Using an ambisense coding strategy, LASV genome encodes four proteins: glycoprotein complex (GPC), nucleoprotein (NP), matrix protein (Z), and the L RNA-dependent RNA polymerase. Instead, these viruses steal the caps from host mRNAs in a process termed cap snatching. In arenaviruses, mutagenesis studies have revealed that the N-terminal domain of the LASV L protein, which consists of 250 amino acid residues, is uniquely required for viral transcription but not replication, implicating its potential role in cap snatching. Our work confirms that arenavirus L polymerase proteins contain a conserved endonuclease domain at the N-terminal region.

Toward this end, we report here for the first time the crystal structure of the endonuclease domain of the LASV L protein in complex with Mg2+ ions at 1.72 Å and demonstrate its enzymatic activity required for viral RNA transcription. The final protein product for crystallization consists of residues 1–173 based on the structure determined. The protein contains an N-terminal domain that consists of a four α-helices bundle (α1, α2, α3 and α7) and a C-terminal domain that composes of three antiparallel β-sheets (β1, β2 and β3) and two helices (α4 and α5). Between the two domains is a highly positively charged groove, which we speculate to be a RNA binding site, and a highly negatively charged cavity, which harbors two magnesium ions (Mg2+) and is a potential active site of the endonuclease domain. Two Mg2+ ions, presumably picked up by the protein from the crystallization solution, are located at the presumed active site of the LASV endonuclease domain. Four water molecules (Wat1, 2, 3 and 4) and the side chain of D89 coordinate the first Mg2+, while three water molecules (Wat4, 5 and 6), the side chain of D89 and the main chain oxygen of C103 coordinate the second Mg2+. This metal binding feature is different from that of the known structures of the influenza and LACV endonucleases, in which both metal ions are coordinated by four or three potential catalytic residues or by residue E80 and three water molecules. In addition to D89, which coordinates the two Mg2+ ions, some other potential catalytic residues are E51 that coordinates Wat1 and Wat6, E102, which is 4.2 Å away from Wat4, D119, which is 5.2 Å from Wat5, K122, which is 5.7 Å from Wat3 and 5.8 Å from the first Mg2+, and H62, which interacts with E51 through side chains and is 6.2 Å away from Wat1. Structural comparison demonstrates that LASV L endonuclease closely resembles the L endonuclease of LCMV with rmsd of 1.382 Å over 166 Cα atoms. However, we notice that the active sites form a deep cavity in PA endonuclease but a flat surface in LASV endonuclease domain, which may partly explain our failure to obtain the LASV L in complex with single ribonucleotides despite multiple attempts.

> GAMADIGSMEEDIACVKDLVSKYLVDNERLSRQKLAFLVQTEPRMLLMEGLKLLSLCIEVDSCNANGCEHNSEDKSVERILHDHGILTPSLCFVVPDGYKLTGNVLILLECFVRSSPANFEQKYIEDFKKLEQLKEDLKSVDINLIPLIDGRTSFYNEQIPDWVNDKLRDTLFSLLKY> MSASRKTLVVTNDFPPRIGGIQSYLRDFIATQDPESIVVFASTQNAEEAHAYDKTLDYEVIRWPRSVMLPTPTTAHAMAEIIREREIDNVWFGAAAPLALMAGTAKQAGASKVIASTHGHEVGWSMLPGSRQSLRKIGTEVDVLTYISQYTLRR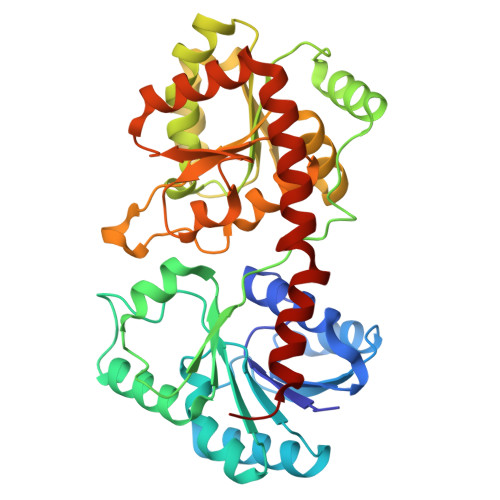FKSAFGSHPTFEHLPSGVDVKRFTPATPEDKSATRKKLGFTDTTPVIACNSRLVPRKGQDSLIKAMPQVIAARPDAQLLIVGSGRYESTLRRLATDVSQNVKFLGRLEYQDMINTLAAADIFAMPARTRGGGLDVEGLGIVYLEAQACGVPVIAGTSGGAPETVTPATGLVVEGSDVDKLSELLIELLDDPIRRAAMGAAGRAHVEAEWSWEIMGERLTNILQSEPR Mitochondrial proteins CHCHD10 and CHCHD2 are mutated in rare cases of heritable FTD, ALS and PD and aggregate in tissues affected by these diseases. Here, we demonstrate that the low complexity N-terminal domains of both D10 and D2, as well as the full-length proteins, can form amyloid fibrils in vitro and in vivo. Structures of D10 and D2 fibrils assembled in vitro from the low complexity N-terminal domains of each protein show that their core comprises the most highly conserved region between the two proteins. For D10 and D2, the central conserved VAV motif forms a beta-strand that is associated with the protofilament interface in all the structures we have observed, suggesting that it may be a critical element in fibril formation and may be expected to appear in ex vivo structures as well.

D2 also features disease-linked mutations in the region constituting the core of D2-NT fibrils. Notably, the most commonly reported pathogenic D2 mutation p.T61I33 occurs at a position facing the interior of the D2 PF fold, suggesting that this mutation, too, could promote alternative fibril structures. To assess this, we solved the structure of T61I D2-NT fibrils to 3.09 Å resolution. These fibrils featured a novel PF fold, consisting of residues G54–G87, that differs from the WT D2-NT fold, all three WT D10-NT folds, and the S59L D10-NT fold. In addition, the T61I PF fold appears to contain several LARKS (low complexity aromatic-linked kinked segments), likely stemming from three glycine-aromatic dipeptides (G59–H60, G63–H64, and G69–F70). Unlike the case of S59L, the T61I mutation does not flip the larger isoleucine sidechain to the PF fold exterior. However, the two valines in the VAV motif, which are found at the PF interface in all other protofilament structures we have observed, are flipped towards the PF interior in the T61I fold. In contrast, the aggregation rates of the T61I D2 mutant did not result in substantial alteration of the aggregation kinetics of D2-NT or appreciable signal loss in NMR spectra. However, the T61I mutation in D2, which also incorporates a large hydrophobic residue, did not result in substantial changes to the aggregation kinetics of the protein or in appreciable signal loss in NMR spectra, indicating that other factors beyond hydrophobicity influence aggregation kinetics.

>MPRGSRSRTSRMAPPASRAPQMRAAPRPAPVAQPPAAAPPSAVGSSAAAPRQPGLMAQMAITAAGVAVGSAVGHTLGHAITGGFSGGSNAEPARPDITYQEPQGTQPAQQQQPM[18x]4-methyl-~{N}-[4-[(4-methylpiperazin-1-yl)methyl]-3-(trifluoromethyl)phenyl]-3-[(1-methyl-6-pyridin-3-yl-pyrazolo[3,4-d]pyrimidin-4-yl)amino]benzamide | C32 H32 F3 N9 O | 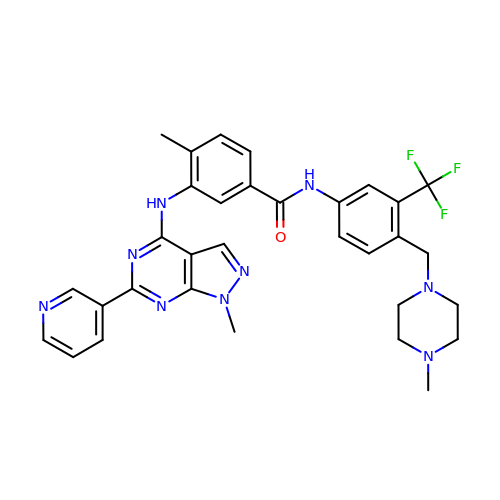ILZAZQWZEHBYCH-UHFFFAOYSA-N> MFPKALGYVTGDMKELANQLKDKPVVLQFIDWILRGISQVVFVNNPVSGILILVGLLVQNPWWALTGWLGTVVSTLMALLLSQDRSLIASGLYGYNATLVGVLMAVFSDKGDYFWWLLLPVCAMSMTCPIFSSALNSVLSKWDLPVFTLPFNMALSMYLSATGHYNPFFPAKLVIPITTAPQISWSDLSALELLKSIPVGVGQIYGCDNPWTGGIFLGAILLSSPLMCLHAAIGSLLGIAAGLSLSAPFENIYFGLWGFNSSLACIAMG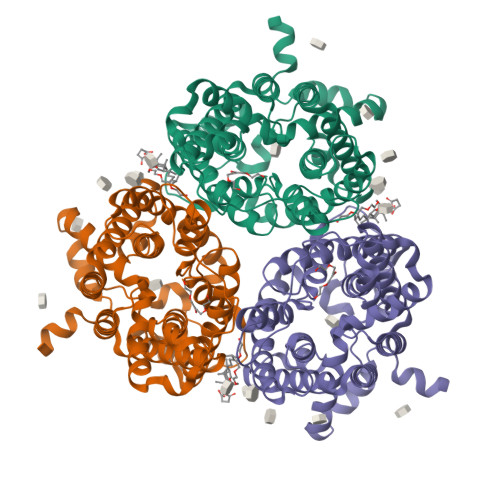GMFMALTWQTHLLALGCALFTAYLGVGMANFMAEVGLPACTWPFCLATLLFLIMTTKNSNIYKMPLSKVTYPEENRIFYLQAKKRMVESPLAENLYFQ>FDFNIMVVGQSGLGKSTLVNTLFKSQVSRKASSWNREEKIPKTVEIKAIGHVIEEGGVKMKLTVIDTPGFGDQINNENCWEPIEKYINEQYEKFLKEEVNIARKKRIPDTRVHCCLYFISPTGHSLRPLDLEFMKHL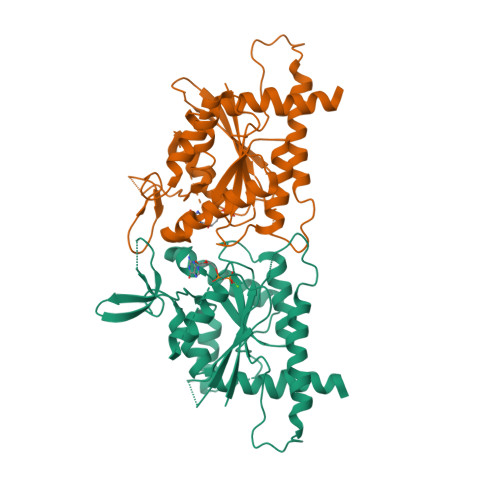SKVVNIIPVIAKADTMTLEEKSEFKQRVRKELEVNGIEFYPQKEFDEDLEDKTENDKIRQESMPFAVVGSDKEYQVNGKRVLGRKTPWGIIEVENLNHCEFALLRDFVIRTHLQDLKEVTHNIHYETYRAKRL[2x]>GPAVRTIRIYQPGEYQPGQLLELSPEAGQHVGVVLRMEQGEQLTLFNGDNKEFTASIERVKKKQVFVRIASVLEVNRESPLKIHLAQAISKGERMEMVMQKSAELGVACITPLITERCQVKIDKEKMAKKMHQWLNIIIGACEQCGRNQIPELRQPVYLDQFVREAKEHLKLILHPAFSKTWRDYPVQPPDVALIIGPEGGFSDEEIRLTSGHGFLPLSLGPRVLRTETAAITALSVLQAAGGDL[4x]

The methylation of U1498 located in the 16S ribosomal RNA of Escherichia coli is an important modification affecting ribosomal activity. RsmE methyltransferases methylate specifically this position in a mechanism that requires an S‐adenosyl‐L‐methionine (AdoMet) molecule as cofactor. The protein comprises an N‐terminal PUA domain and a C‐terminal SPOUT domain. The latter is responsible for protein dimerization and cofactor binding.

Here we report the structure of Apo and AdoMet‐bound Lpg2936 from Legionella pneumophila at 1.5 and 2.3 Å, respectively. Comparison with similar structures suggests that Lpg2936 is an RsmE‐like enzyme that can target the equivalent of U1498 in the L. pneumophila ribosomal RNA, thereby potentially enhancing ribosomal activity during infection‐mediated effector production. The multiple copies of the enzyme found in both structures reveal a flexible conformation of the bound AdoMet ligand.> PQFGLFSKYRTPNCRRYSIHGCNRMYAPVCGSDMSTYANECTLCMKIREGGHN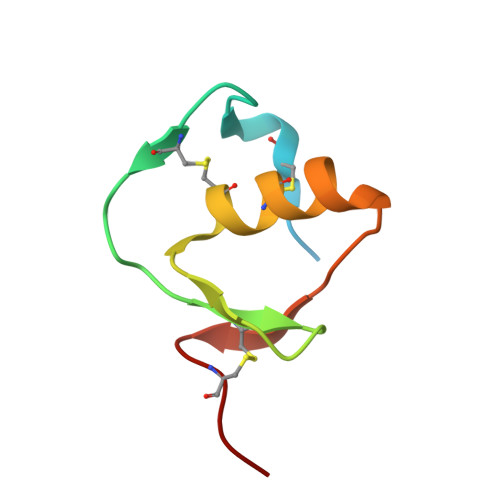IKIIKNGPCGAS>[2x]MTAHRSVLLVVHTGRDEATETARRVEKVLGDNKIALRVLSAEAVDRGSLHLAPDDMRAMGVEIEVVD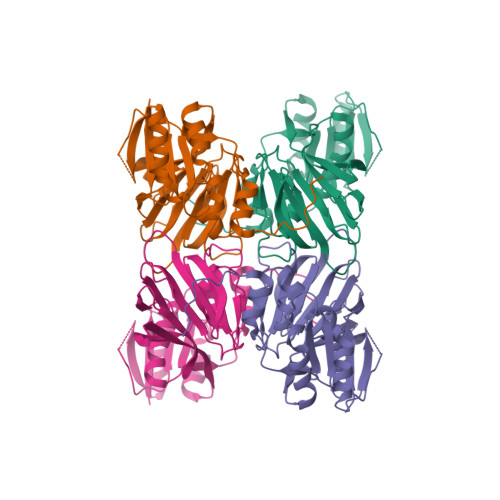ADQHAADGCELVLVLGGDGTFLRAAELARNASIPVLGVNLGRIGFLAEAEAEAIDAVLEHVVAQDYRVEDRLTLDVVVRQGGRIVNRGWALNEVSLEKGPRLGVLGVVVEIDGRPVSAFGCDGVLVSTPTGSTAYAFSAGGPVLWPDLEAILVVPNNAHALFGRPMVTSPEATIAIEIEADGHDALVFCDGRREMLIPAGSRLEVTRCVTSVKWARLDSAPFTDRLVRKFRLPVIGWRGK> CAAELAALEAELAALEGHVEEADFP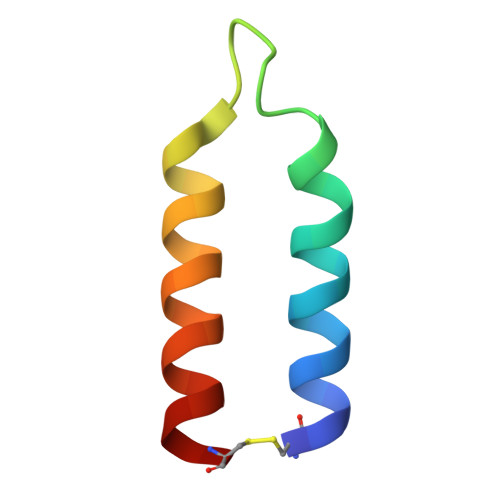WGKLNNLIEKLWQLKQACX>[4x]EPEITLIIFGVIAGVIGTILL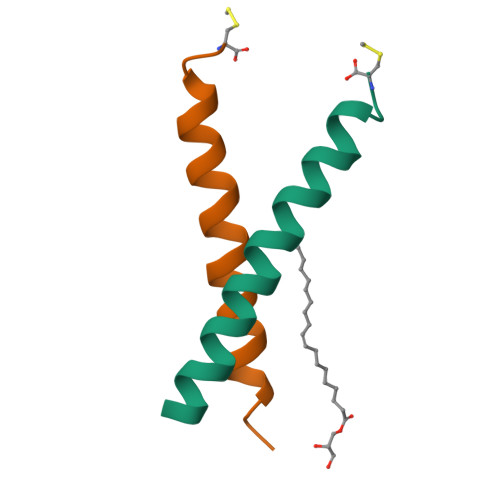ISYGIRRLC>GSSTTFAARLNRLFDTVYPPGRGPHTSAEVIAALKAEGITMSAPYLSQLR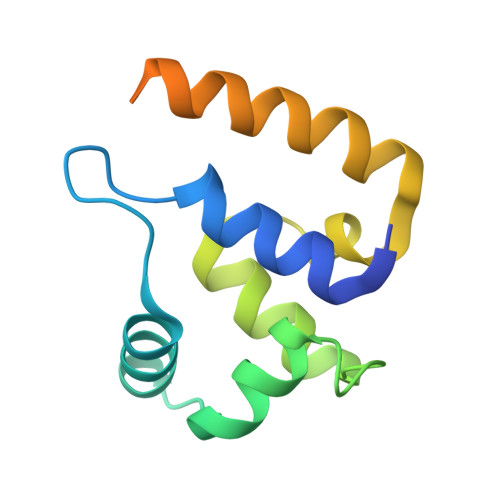SGNRTNPSGATMAALANFFRIKAAYFTDDEYYEKLDKELQWLCTMRDDGVRRIAQRAHGLPSAAQQKVLDRID[2x]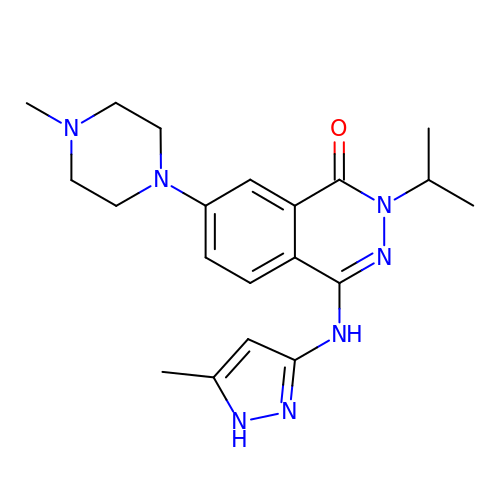7-(4-methylpiperazin-1-yl)-4-[(5-methyl-1H-pyrazol-3-yl)amino]-2-(propan-2-yl)phthalazin-1(2H)-one | C20 H27 N7 O | VLOGKAVNBJBYON-UHFFFAOYSA-N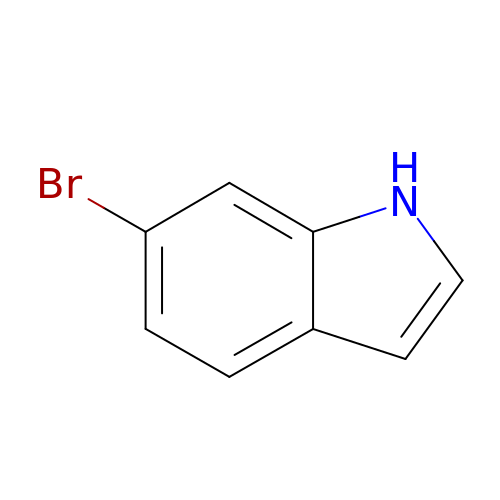6-bromo-1H-indole | C8 H6 Br N | MAWGHOPSCKCTPA-UHFFFAOYSA-N Versatile peroxidase (VP, EC 1.11.1.16) constitutes the third family of ligninolytic peroxidases, which was described 20-years ago. VP combines catalytic properties of the above two families due to the presence of both a Mn-oxidation site and a catalytic tryptophan in its molecular structure. In the present work, VP (isoenzyme VPL2) from Pleurotus eryngii has been subjected to protein engineering using a rational design strategy.

A third approach to improve the stability of VP was the further structural stabilization of the distal Ca2+-binding site, responsible for maintaining the relative position of the distal histidine involved in enzyme activation by H2O2. For that, the VPi-ss variant was designed by adding a double mutation (A49C/A61C) to VPi. The two cysteines added to this variant should form an extra disulfide bond contributing to the structural stabilization of the loop containing two of the four amino acid residues that coordinate the distal Ca2+ ion. Finally, the VPi-ss structure confirmed that the two cysteines introduced at positions 49 and 61 form an extra (fifth) disulfide bond next to the distal Ca2+ binding site. This region did not show any additional change compared with the native enzyme even though the two new cysteines occupy positions adjacent to Asp48, Gly60, Asp62 and Ser64 involved, together with two water molecules, in Ca2+ coordination. VPi-br harboring seven additional basic residues exposed to the solvent, and VPi-ss containing two cysteines added to form an additional extra disulfide bond, further improved the stability of VPi at acidic pH (respectively). Both variants retained 86% and 85% of the initial activity at pH 3.5 after 24 h of incubation compared to the 61% retained by VPi and far from the 1% of the native VP. In short, the extra disulfide bond contributes to stabilize the position of the distal histidine in helix B. This analysis, together with that previously performed for VPi, could explain the accumulative effect due to this disulfide bond and the extra hydrogen bond and salt bridge interactions on the VPi-ss stability improvement observed at pH 3.5. However, VPi-ss did not show increased stability at neutral pH compared with VPi, unlike what was observed at pH 3.5.

> AKCDDGRTTANAACCILFPILDDIQENLFDGAQCGEEVHESLRLTFHDCIGFSPTLGGGGCDGSIIAFSDIETNFPANAGIDEIVEAQKPFVAKHNISAGDFIQFAGAVGVSNCPGGVRIPFFLGRPDAVKASPDHLVPEPFDSVTSILARMGDAGFSPVEVVWLLASHSIAAADKVDPSIPGTPFDSTPGVFDSQFFIETLLKGRLFPGTADNKGEAQSPLQGEIRLQSDELLARDPRTACEWQSMVNNQPKIQNRFAATMSKMALLGQDKTKLIDCSDVIPTPPALVGAAHLPAGFSLKDVEQACRKTPFPRLTADPGPVTSVPPVPGS> QEVEFDIPPQALGSALQEFGRQADIQVLYRPEEVRNKRSSAIKGKLEPNQAITELLRGTGASVDFQGNAITISVAEAADSSVDLGATMITSNQLGTITEDSGSYTPGTIATATRLVLTPRETPQSITVVTRQNMDDFGLNNIDDVMRHTPGITVSAYDTDRNNYYARGFSINNFQYDGIPSTARNVGYSAGNTLSDMAIYDRVEVLKGATGLLTGAGSLGATINLIRKKPTHEFKGHVELGAGSWDNYRSELDVSGPLTESGNVRGRAVAAYQDKHSFMDHYERKTSVYYGILEFDLNPDTMLTVGADYQDNDPKGSGWSGSFPLFDSQGNRNDVSRSFNNGAKWSSWEQYTRTVFANLEHNFANGWVGKVQLDHKINGYHAPLGAIMGDWPAPDNSAKIVAQKYTGETKSNSLDIYLTGPFQFLGREHELVVGTSASFSHWEGKSYWNLRNYDNTTDDFINWDGDIGKPDWGTPSQYIDDKTRQLGSYMTARFNVTDDLNLFLGGRVVDYRVTGLNPTIRESGRFIPYVGAVYDLNDTYSVYASYTDIFMPQDSWYRDSSNKLLEPDEGQNYEIGIKGEYLDGRLNTSLAYFEIHEENRAEEDALYNSKPTNPAITYAYKGIKAKTKGYEAEISGELAPGWQVQAGYTHKIIRDDSGKKVSTWEPQDQLSLYTSYKFKGALDKLTVGGGARWQGKSW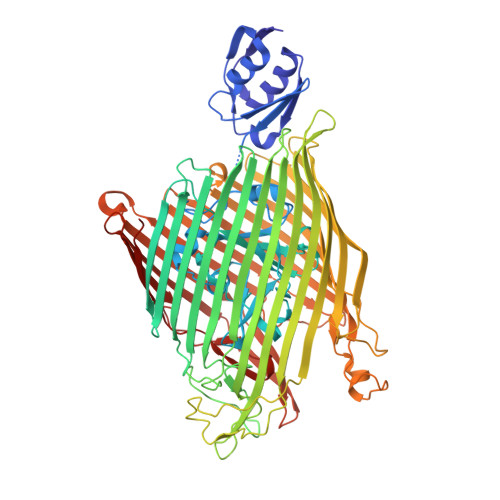QMVYNNPRSRWEKFSQEDYWLVDLMARYQITDKLSASVNVNNVFDKTYYTNIGFYTSASYGDPRNLMFSTRWDF>[3x]MHHHHHHENL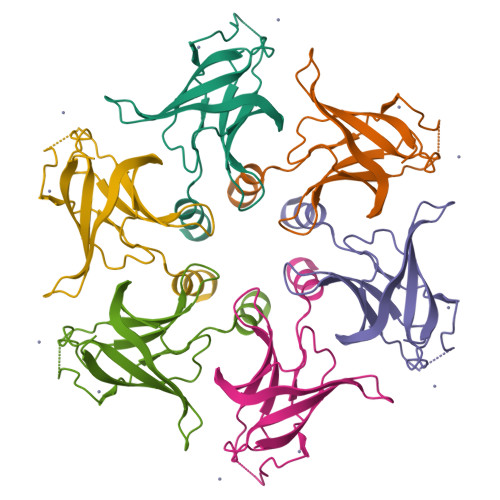YFQTSIRTEPTYTLYATFDNIGGLKARSPVSIGGVVVGRVADITLDPKTYLPRVTLEIEQRYNHIPDTSSLSIRTSGLLGEQYLALNVGFEDPELGTAILKDGDTIQDTKSAMVLEDLIGQFLYGSKGDDNKNSGDAPAAAPGNNETTEPVGTTK> GWEKDLEEALEAGGCDLETLRNIIQGRPLPADLRAKVWKIALNVAGKGDSLASWDGILDLPEQNTIHKDCLQFIDQLSVPEEKAAELLLDIESVITFYCKSRNIKYSTSLSWIHLLKPLVHLQLPRSDLYNCFYAIMNKYIPRDCSQKGRPFHLFRLLIQYHEPELCSYLDTKKITPDSYALNWLGSLFACYCSTEVTQAIWDGYLQQADPFFIYFLMLIILVNAKEVILTQESDSKEEVIKFLENTPSSLNIEDIEDLFSLAQYYCSKTPASFRKDNHHLFGSTLLGIKDDDADLSQ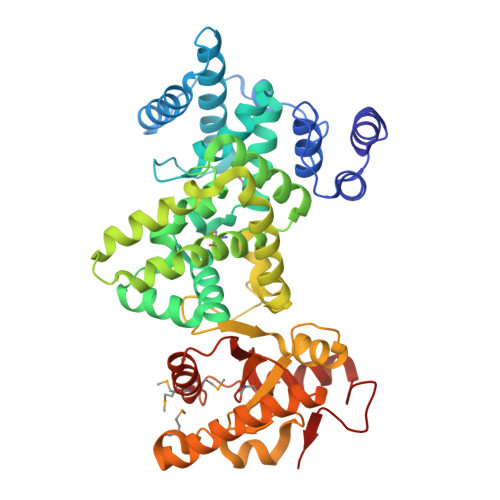ALCLAISVSEILQANQLQGEGVRFFVVDCRPAEQYNAGHLSTAFHLDSDLMLQNPSEFAQSVKSLLEAQKQSIESGSIAGGEHLCFMGSGREEEDMYMNMVLAHFLQKNKEYVSIASGGFMALQQHLADINVDGPENGYGHWIAST N-[(6-methylimidazo[1,2-a]pyridin-2-yl)methyl]-4-oxidanylidene-pyrido[1,2-a]pyrimidine-2-carboxamide 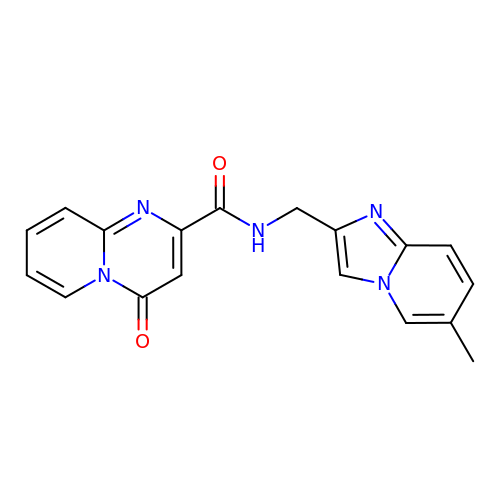| C18 H15 N5 O2 | HGTYDECGVDYGCR-UHFFFAOYSA-N> ETGSLYLWIDAHQARVLIGFEEDILIVSEGKMAPFTHDFRKAQQRMPAIPVNIHSMNFTWQAAGQAEYFYEFLSLRSLDKGIMADPTVNVPLLGTVPHKASVVQVGFPCLGKQDGVAAFEVDVIVMNSEGNTILKTP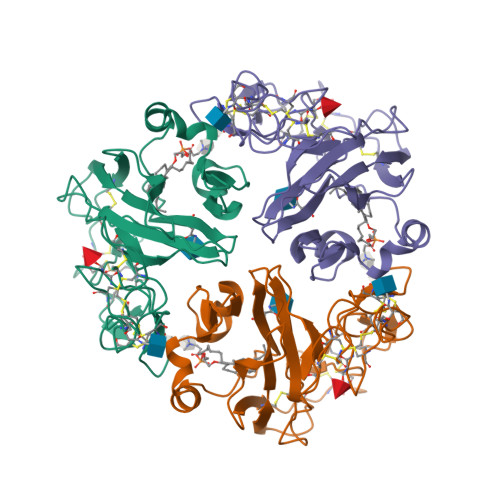QNAIFFKTCQQAECPGGCRNGGFCNERRICECPDGFHGPHCEKALCTPRCMNGGLCVTPGFCICPPGFYGVNCDKANCSTTCFNGGTCFYPGKCICPPGLEGEQCEISKCPQPCRNGGKCIGKSKCKCSKGYQGDLCSKPVCEPGCGAHGTCHEPNKCQCQEGWHGRHCNKRYEASLIGTKHHHHHH> GPVHINKGGRPRQHLLSLTRRAQKHRLRELKIQVKEFADKEEGGDVKAVCLTLFLLALRARNEHRQADELEAIMQGRGSGLQPAVCLAIRVNTFLSCSQYHKMYRTVKAITGRQIFQPLHALRNAEKVLLPGYHPFEWQPPLKNVSSRTDVGIIDG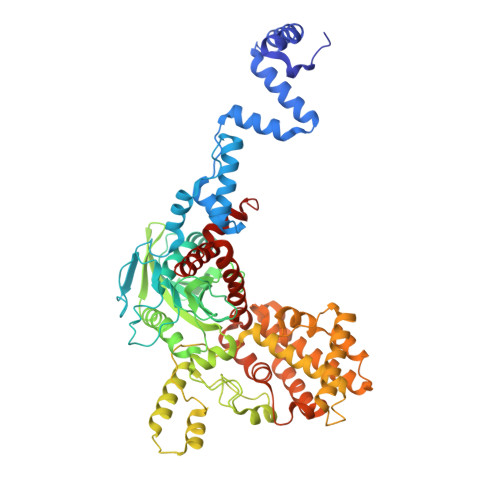LSGLASSVDEYPVDTIAKRFRYDSALVSALMDMEEDILEGMRSQDLDDYLNGPFTVVVKESCDGMGDVSEKHGSGPAVPEKAVRFSFTVMRITIEHGSQNVKVFEEPKPNSELCCKPLCLMLADESDHETLTAILSPLIAEREAMKSSELTLEMGGIPRTFKFIFRGTGYDEKLVREVEGLEASGSVYICTLCDTTRLEASQNLVFHSITRSHAENLQRYEVWRSNPYHESVEELRDRVKGVSAKPFIETVPSIDALHCDIGNAAEFYKIFQLEIGEVYKHPNASKEERKRWQATLDKHLRKRMNLKPIMRMNGNFARKLMTQETVDAVCELIPSEERHEALRELMDLYLKMKPVWRSSCPAKECPESLCQYSFNSQRFAELLSTKFKYRYEGKITNYFHKTLAHVPEIIERDGSIGAWASEGNESGNKLFRRFRKMNARQSKCYEMEDVLKHHWLYTSKYLQKFMNAHNA> GSSMKC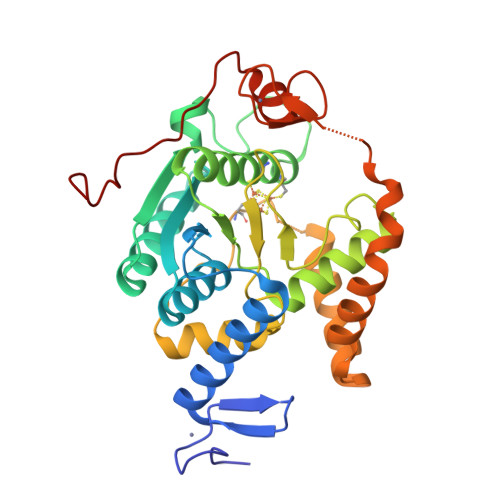KFCSREAYIKIHYPKMYLCEEHFKEYFERKVSRTIERYKLLTKDERILVAVSGGKDSAVTAYVLKKLGYNIECLHINLGISGYSEKSEEYAKKQCKLIGAPLHIVRIKEILGYGIGEVKTRRPPCSYCGLTKRYIMNKFAYDNGFDAIATGHNLDDEASFLLNNILHWNTEYLAKGGPILPQQGKFIKKVKPLYEVTEREVVAYALAVGLEYIVEECPYARGATTLDMKGVLNELEEKRPGTKFNFVRGYLKKKKLFEPEIKEKEIKECKICRMPSSGDICAFCKFWGLKKEINFKVSSTDEEPFGP> DQQLVDQLSQLKLNVKMLDNRAGENGVDCAALGADWASCNRVLFTLSNDGQAIDGKDWVIYFHSPRQTLRVDNDQFKIAHLTGDLYKLEPTAKFSGFPAGKAVEIPVVAEYWQLFRNDFLPRWYATSGDAKPKMLANTDTENLDQFVAPFTGDQWKRTKDDKNILMTPASRFVSNADLQTLPAGALRGKIVPTPMQVKVHAQDADLRKGVALDLSTLVKPAADVVSQRFALLGVPVQTNGYPIKTDIQPGKFKGAMAVSGAYELKIGKKEAQVIGFDQAGVFYGLQSILSLVPSDGSGKIATLDASDAPRFPYRGIFLDVARNFHKKDAVLRLLDQMAAYKLNKFHFHLSDDEGWRIEIPGLPELTEVGGQRCHDLSETTCLLPQYGQGPDVYGGFFSRQDYIDIIKYAQARQIEVIPEIDMPAHARAAVVSMEARYKKLHAAGKEQEANEFRLVDQTDTSNTTSVQFFNRQSYLNPCLDSSQRFVDKVIGEIAQMHKEAGQPIKTWHFGGDDAKNIRLGAGYTDKAKPEPGKGIIDQSNEDKPWAKSQVCQTMIKEGKVADMEHLPSYFGQEVSKLVKAHGIDRMQAWQDGLKDAESSKAFATSRVGVNFWDTLYWGGFDSVNDWANKGYEVVVSNPDYVYMDFPYEVNPDERGYYWGTRFSDERKVFSFAPDNMPQNAETSVDRDGNHFNAKSDKPWPGAYGLSAQLWSETQRTDPQMEYMIFPRALSVAERSWHRAGWEQDYRAGREYKGGETHFVDTQALEKDWLRFANILGQRELAKLDKGGV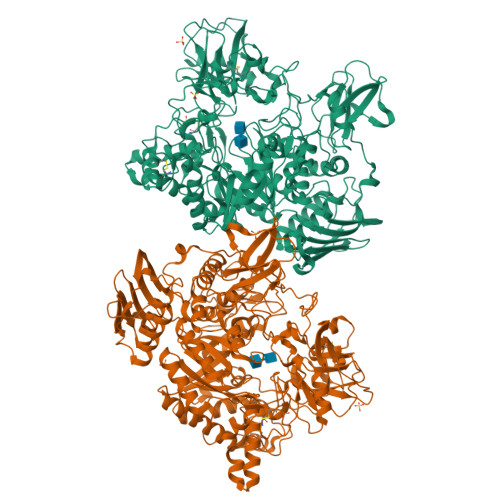AYRLPVPGARVAGGKLEANIALPGLGIEYSTDGGKQWQRYDAKAKPAVSGEVQVRSVSPDGKRYSRAEKV>MNHKVHHHHHHMGGGSTPLPLPQQQPPQQEPPPPPVPLASRAACEALKDGNGDMVWPNAATVVEVAAWRDAAPATASAAALPEHCEVSGAIAKRTGIDGYPYEIKFRLRMPAEWNGRFFMEGGSGTNGSLSAATGSIGGGQIASALSRNFATIATDGGHDNAVNDNPDALGTVAFGLDPQARLDMGYNSYDQVTQAGKAAVARFYGRAADKSYFIGCSEGGREGMMLSQRFPSHYDGIVAGAPGYQLPKAGISGAWTTQSLAPAAVGLDAQGVPLINKSFSDADLHLLSQAILGTCDALDGLADGIVDNYRACQAAFDPATAANPANGQALQCVGAKTADCLSPVQVTAIKRAMAGPVNSAGTPLYNRWAWDAGMSGLSGTTYNQGWRSWWLGSFNSSANNAQRVSGFSARSWLVDFATPPEPMPMTQVAARMMKFDFDIDPLKIWATSGQFTQSSMDWHGATSTDLAAFRDRGGKMILYHGMSDAAFSALDTADYYERLGAAMPGAAGFARLFLVPGMNHCSGGPGTDRFDMLTPLVAWVERGEAPDQISAWSGTPGYFGVAARTRPLCPYPQIARYKGSGDINTEANFACAAPP[6x]

Recently, the bacterial strain Ideonella sakaiensis 201-F6 was discovered and shown to grow on low-crystallinity PET films. Two α/β-hydrolase fold enzymes (α/β-hydrolases), PETase and MHETase, work together to degrade PET in two steps via MHET, yielding TPA and ethylene glycol—the building blocks required for a new round of PET synthesis. We have determined crystal structures of recombinantly expressed and purified I. sakaiensis MHETase in its ligand-free form (2.05 Å resolution), MHETase bound to a nonhydrolyzable mono-(2-hydroxyethyl) terephthalamide (MHETA, 2.1 Å resolution) or to benzoic acid (BA, 2.2 Å resolution) as well as ligand-free PETase (2.0 Å resolution) (2a−f). PETase and MHETase only share the α/β-hydrolase fold (2.87 Å RMSD for 184 out of 262 residues aligned).

Apart from the entire substrate, even substrate sub-structures and analogs such as benzoic acid or nicotinic acid are able to bind tightly to MHETase as observed in the respective co-structure and in differential scanning fluorimetry (DSF) measurements. It is again mainly lid domain residues, which establish the contacts to benzoic acid and place it in an identical position as MHETA. Thus, substrate recognition strongly relies on the aromatic ring as well as the carboxylate function of MHET both guiding its positioning for hydrolysis. Inhibitor experiments with benzoate derivatives and R411 and S416 mutants also demonstrate the importance of the interaction between the carboxylate moiety of the ligand and R411 together with hydrogen bonding for tight binding. Consequently, the loss of the positive charge in the MHETase R411Q and R411A variants leads to strongly reduced substrate binding and decreased inhibition by benzoate in mono-4-nitrophenyl terephthalate (MpNPT) hydrolysis. The high affinity for compounds with a benzoate substructure is expected to lead to product inhibition by formed TPA when higher concentrations of MHET are hydrolyzed in vitro. This is demonstrated by the decreasing reaction rate for MHET hydrolysis over time. The effect of product inhibition is likely less pronounced in the natural environment where formed TPA is metabolized by the bacterium.>[2x]GPGSNEFYLKTWSEWEKNGTPGEQRNIAFNRLKIC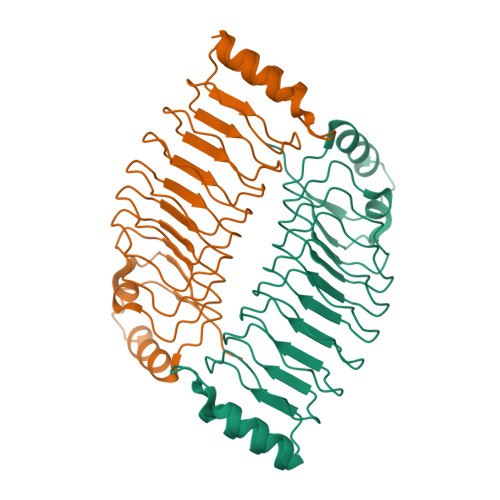LQNQEAELNLSELDLKTLPDLPPQITTLEIRKNLLTHLPDLPPMLKVIHAQFNQLESLPALPETLEELNAGDNKIKELPFLPENLTHLRVHNNRLHILPLLPPELKLLVVSGNRLDSIPPFPDKLEGLALANNFIEQLPELPFSMNRAVLMNNNLTTLPESVLRLAQNAFVNVAGNPLSGHTMRTLQQITTGPDYSGPRIFFSMG>[2x]MNTVRSEKDSMGAIDVPADKLWGAQTQRSLEHFRISTEKMPTSLIHALALTKRAAAKVNEDLGLLSEEKASAIRQAADEVLAGQHDDEFPLAIWQTGSGTQSNMNM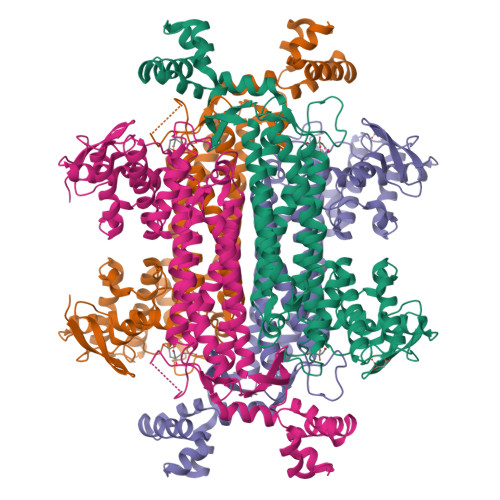NEVLANRASELLGGVRGMERKVHPNDDVNKSQSSNDVFPTAMHVAALLALRKQLIPQLKTLTQTLNEKSRAFADIVKIGRTHLQDATPLTLGQEISGWVAMLEHNLKHIEYSLPHVAELALGGTAVGTGLNTHPEYARRVADELAVITCAPFVTAPNKFEALATCDALVQAHGALKGLAASLMKIANDVRWLASGPRCGIGEISIPENQPGSSIMPGKVNPTQCEALTMLCCQVMGNDVAINMGGASGNFELNVFRPMVIHNFLQSVRLLADGMESFNKHCAVGIEPNRERINQLLNESLMLVTALNTHIGYDKAAEIAKKAHKEGLTLKAAALALGYLSEAEFDSWVRPEQMVGSMKAGR> MGHHHHHHMLHLLEQIRAYCETCWEWQEAHEPGMDQDKNPMPAPVEHQICPAVCVLMKLSFDEEHRHAMNELGGLQAIAELLQVDCEMYGLTNDHYSITLRRYAGMALTNLTFGDVANKATLCSMKGCMRALVAQLKSESEDLQQVIASVLRNLSWR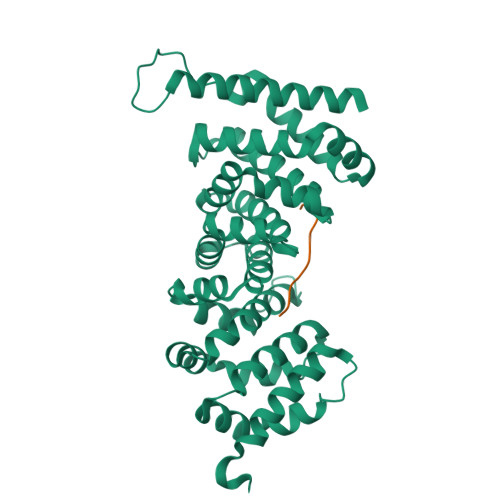ADVNSKKTLREVGSVKALMECALEVKKESTLKSVLSALWNLSAHCTENKADICAVDGALAFLVGTLTYRSQTNTLAIIESGGGILRNVSSLIATNEDHRQILRENNCLQTLLQHLKSHSLTIVSNACGTLWNLSARNPKDQEALWDMGAVSMLKNLIHSKHKMIAMGSAAALRNLMANRPAKYKDANIMSPGSSLPS;> LTGCGDIIAEQ> 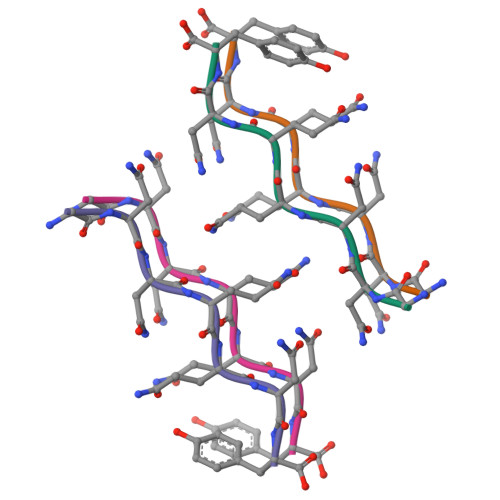GNNQQNY>MSAYQTVVVGTD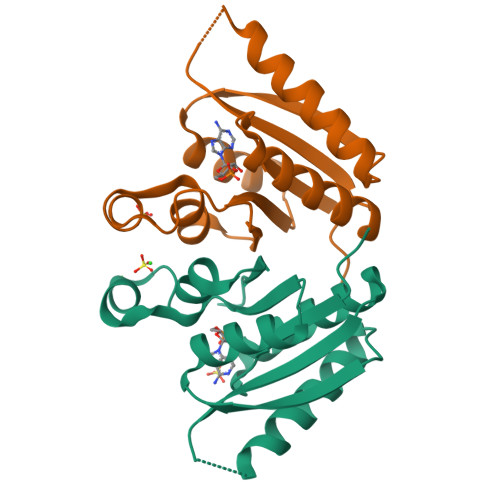GSDSSLRAVDRAGQIAAASNAKLIIATAYFPQSEDSRAADVLKDEGYKMAGNAPIYAILREANDRAKAAGATDIEERPVVGAPVDALVELADEVKADLLVVGNVGLSTIAGRLLGSVPANVARRSKTDVLIVHTS[6x]>GS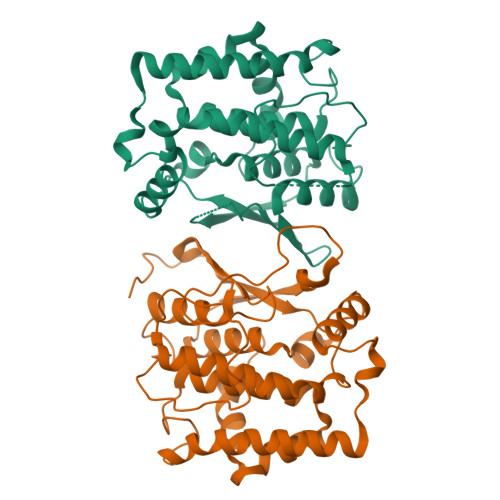MPPTSTTSNPIVFYDIATRPPVEKTCCSPNPWKTRLALNFKDLPYSTSWVALPDISKVRGSLKVPPCRKFADGTDFFTLPIIEDPATDSLVGDSFDIAVYLQKTYPKSGAGDLFPPQSLDYVFKHNGILVPLSECRESEFPEYARFNMNIDAAFTTHTQLTVQGFPFDPATAEATKAEFVRRGGVSCWDDFALVGEQREKMMDSFQNMLGDLAKLFLKDTSGPFLLGTKASYADLMIGAWLRMMHVTLPESEWEEVRSWHEGIFGQLYDALETYAEVK[2x]> TGGRNSIRYSELAPLFDTTRVYLVDNKSTDVASLNYQNDHSNFLTTVIQNNDYSPGEASTQTINLDDRSHWGGDLKTILHTNMPNVNEFMFTNKFKARVMVSRSLTKDKQVELKYEWVEFTLPEGNYSETMTIDLMNNAIVEHYLKVGRQNGVLESDIGVKFDTRNFRLGFDPVTGLVMPGVYTNEAFHPDIILLPGCGVDFTHSRLSNLLGIRKRQPFQEGFRITYDDLEGGNIPALLDVDAYQASLKDDTEQGGDGAGGGNNSGSGAEENSNAA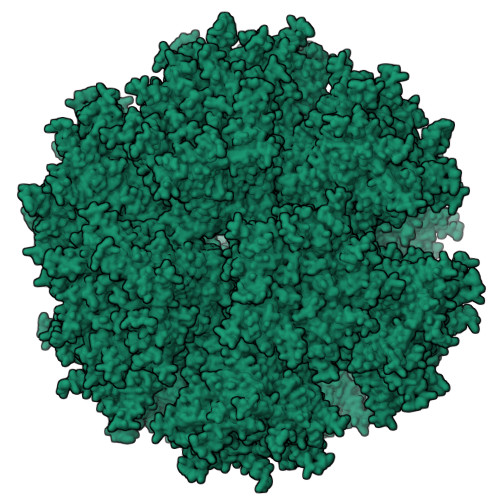AAAMQPVEDMNDHAIRGDTFATRAEEKRAEAEAAAEAAAPAAQPEVEKPQKKPVIKPLTEDSKKRSYNLISNDSTFTQYRSWYLAYNYGDPQTGIRSWTLLCTPDVTCGSEQVYWSLPDMMQDPVTFRSTSQISNFPVVGAELLPVHSKSFYNDQAVYSQLIRQFTSLTHVFNRFPENQILARPPAPTITTVSENVPALTDHGTLPLRNSIGGVQRVTITDARRRTCPYVYKALGIVSPRVLSSRTF> MPSSHHHHHHSQDPNCLIQIPSAKDIQQMHGMPAGADEDQFERLKHMTQVIATTQSKDPSLPVVTTDRVELPEHWNQLFAAMKKGDENVALTLFAEFPEEDQILQALLAVHTSEYLQQIIRDCIQAQAKGWKQLNSDILITPGTFEVLIKDISMTLFHSKKVHFSFGLPTHHAFADEGSGFCILNKSAVLLKHMQRNTKPLKHIIVGTDVNRDNGLCDILMNSAADMDICHIDVFDSRVYPYQDEDYITELFNKCGKDEGQNIQSWQRGGLDYFVVNLSRTTRKPGLVHPALVFAIEKMEEQIEQAKINHQKVALFLPTGWDSHEEETAYCGKYVDGYLMGATEARKTRLNTTDLTYFYESIFKLYRENKDHIEKVYWGLEGGYDRKMYEQQIELLMSIVLN

Classical Zn2+-dependent deac(et)ylases play fundamental regulatory roles in life and are well characterized in eukaryotes regarding their structures, substrates and physiological roles. Structurally, these enzymes are composed of a central eight-stranded parallel β-sheet flanked by α-helices on each site, known as the α/β-arginase/deacetylase fold. All active site residues were conserved, as shown by the multiple sequence alignment and the structural alignment, suggesting a general acid/base catalytic mechanism for the bacterial enzymes as described for the eukaryotic counterparts. These enzymes mediate catalysis using a penta-coordinated catalytic Zn2+ ion coordinated by two aspartates and a histidine (KpHdaH (1b): Asp181, Asp269, His183).

We were able to solve two crystal structure for two Legionella enzymes of cluster 3, L. cherrii ApaH and L. pneumophila ApaH. Structurally, compared to the arginase-deacetylase core, LpApaH and LcApaH contain an additional pair of α-helices and the central parallel β-sheet is extended by a two-stranded antiparallel β-sheet. These features might be needed for recognition of the enzymes by the type IV secretion system for secretion into the host cell, or important for interaction with other proteins such as the methyltransferase RomA or the lysine acetyltransferase KAT7 in the host cells, which calls for further investigations. In LcApaH and LpApaH the XGGY-motif is conserved (LcApaH: 388-EGGY−391/LpApaH: 391-EGGY−394). The RPP-motif is substituted by the motif 176-GLPSHH-181 (LcApaH)/176-GLPSHH-181 (LpApaH), however, with highly similar main-chain traces. To this end, differences in the sequences in the region of the RPP-motif might explain the observed highest activity as deacetylase while also being active as depropionylase and de-d/l-lactylase. For the enzymes LcApaH and LpApaH, we discovered the highest deacetylation efficiency of all compared enzymes with kcat/KM-values of 139 × 103 M−1 s−1 and 75 × 103 M−1 s−1 for the histone H4 peptide LGKac, respectively. LcApaH converts the lactylated peptides LGKd-la and LGKl-la with comparable catalytic efficiency for the two stereoisomers (kcat/KM (Kl-la): 0.03 × 103 M−1 s−1 and kcat/KM (Kd-la): 0.04 × 103 M−1 s−1) but more than three orders of magnitude less efficient than its deacylation of LGKac (kcat/KM (Kac): 139 × 103 M−1 s−1). The structures show an open active site entry due to absence of oligomer formation and, as a consequence, the missing in trans supply of the active site lid as observed for cluster 1 and cluster 4 enzymes. Notably, for the cluster 3 enzymes LpApaH and LcApaH we discovered the highest discrepancy in the inhibitory potency between SAHA and TSA, with TSA inhibiting the enzymes almost 80–95-fold stronger.>[3x]SNAMSTTSSVRLRPLEREDLPFVHQLDNNASIMRYWFEEPYEAFVELCDLYDKHIHDQ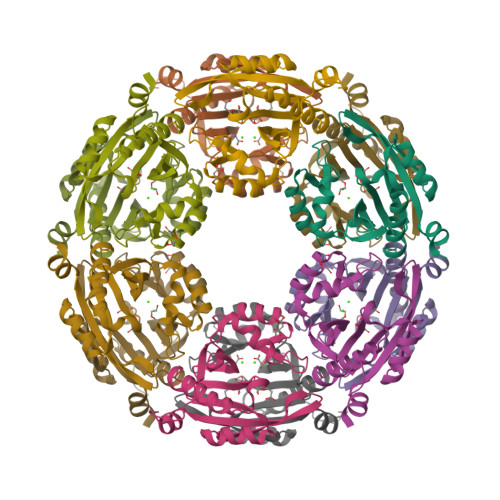SERRFIIESQGTKIGLVELVEINHIHRRAEFQIIIDPTHQGKGYAGAAAKLAMEYGFSVLNLYKLYLIVDKENEKAIHIYSKLGFEIEGELKQEFFINGEYRTVIRMCIFQPQYLAKYKTPSIKNA>MENSFKAALKAGRPQIGLWLGLSSSYSAELLAGAGFDWLLIDGEHAPNNVQTVLTQLQAIAPYPSQPVVRPSWNDPVQIKQLLDVGTQTLLVPMVQNADEAREAVRATRYPPAGIRGVGSALARASRWNRIPDYLQKANDQMCVLVQIETREAMKNLPQILDVEGVDGVFIGPADLSADMGYAGNPQHPEVQAAIEQAIVQIRESGKAPGILIANEQLAKRYLELGALFV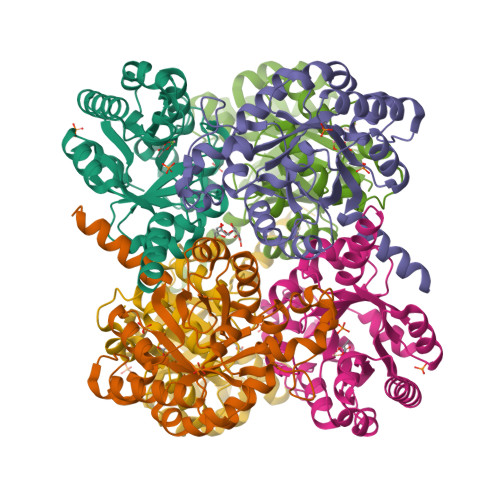AVGVDTTLLARAAEALAARFG[2x]> GSGSGMDEIVKVLSQHDRILVVGHIMPDGDCVSSVLSLTLGLEKLGKEVKAAVDYKIPYVFEKFPYIDKIEENPNFDPELLVVVNASSPDRIGKFQDLLDKVPSVVIDHHSTNTNFGNWNWVDPSFAATAQMIFRINKALGVEYDSNLATLNYLGIATNTGFFRHSNADVRVFEDAYKLVKMGADAHF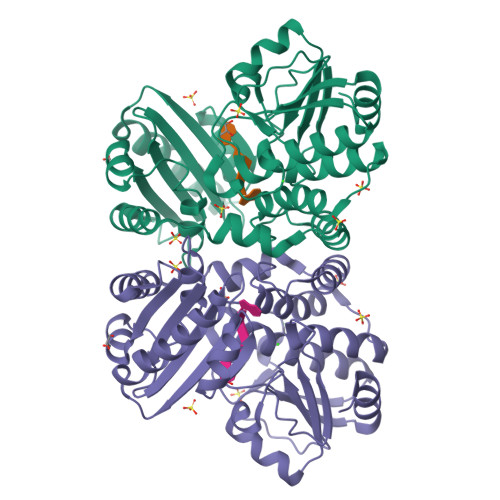VAKEILENKRFEQFKLFAEVLERLQLLENGKIAYSYIDYDTYLRHNCTDEDSAGFVGELRSIRGVEVAVLFMEFPRGKIHVSMRSKDWFNVNEVAFELGGGGHPRAAGVTFEGKKIEEVIPRVINHLLKKFKEGVESESEKIPEGDVLGG>PEIITPIITPFTKDNRIDKEKLKIHAENLIRKGIDKLFVNGTTGLGPSLSPEEKLENLKAVYDVTNKIIFQVGGLNLDDAIRLAKLSKDFDIVGIASYAPYYYPRMSEKHLVKYFKTLCEVSPHPVYLYNYPTATGKDIDAKVAKEIGCFTGVKDTIENIIHTLDYKRLNPNMLVYSGSDMLIATVASTGLDGNVAAGSNYLPEVTVTIKKLAMERKIDEALKLQFLHDEV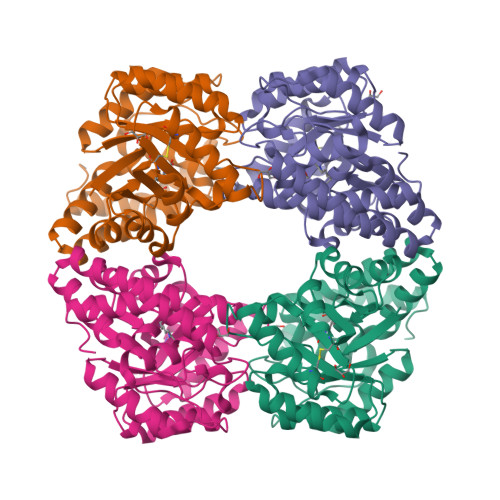IEASRIFGSLSSNYVLTKYFQGYDLGYPRPPIFPLDDEEERQLIKKVEGIRAKLVELKILKE[4x]>[2x]STGPVAPLPTPPNFPNDIALFQQAYQNWSKEIMLDATWVCSPKTPQDVVRLANWAHEHDYKIRPRGAMHGWTPLTVEKGANVEKVILADTMTHLNGITVNTGGPVATVTAGAGASIEAIVTELQKHDLGWANLPAPGVLSIGGALAVNAHGAALPAVGQTTLPGHTYGSLSNLVTELTAVVWNGTTYALETYQRNDPRITPLLTNLGRCFLTSVTMQAGPNFRQRCQSYTDIPWRELFAPKGADGRTFEKFVAESGGAEAIWYPFTEKPWMKVWTVSPTKPDSSNEVGSLGSAGSLVGKPPQAREVSGPYNYIFSDNLPEPITDMIGAINAGNPGIAPLFGPAMYEIT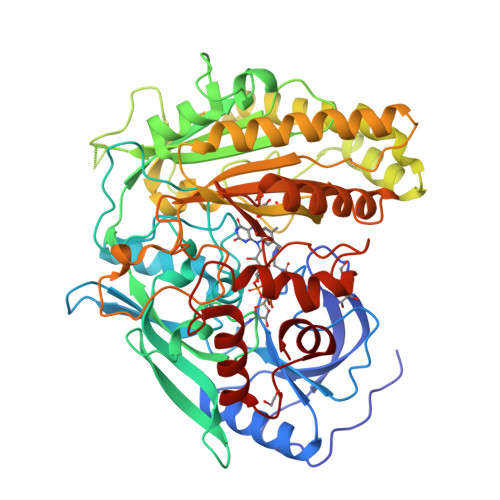KLGLAATNANDIWGWSKDVQFYIKATTLRLTEGGGAVVTSRANIATVINDFTEWFHERIEFYRAKGEFPLNGPVEIRCCGLDQAADVKVPSVGPPTISATRPRPDHPDWDVAIWLNVLGVPGTPGMFEFYREMEQWMRSHYNNDDATFRPEWSKGWAFGPDPYTDNDIVTNKMRATYIEGVPTTENWDTARARYNQIDPHRVFTNGFMDKLLP> MLKQVEIFTDGSCLGNPGPGGYGAILRYRGREKTFSAGYTRTTNNRMELMAFIVALEALKEHCEVILSTDSQYVRQGITQWIHNWKKRGWKTADKKPVKNVDLWQRLDA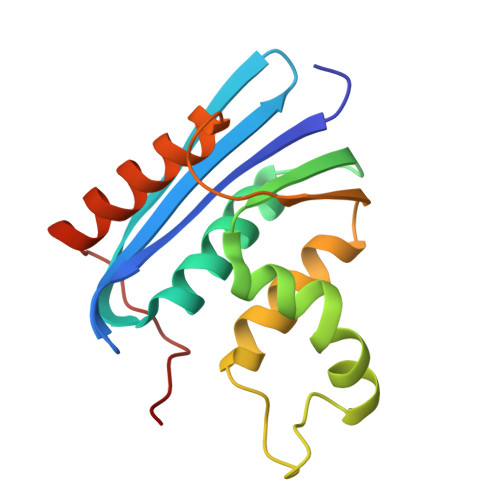ALGQHQIKWEWVKGHAGHPENERCDELARAAAMNPTLEDTGYQVEV>[4x]MKPLLSGSIPVEQFVQTLEKHGFSDIKVEDTAKGHIVLLQEAETLIQIEEDSTHIICDNDEMLRVRLRDLVLKFLQKF;>GSHMRLVSSEQA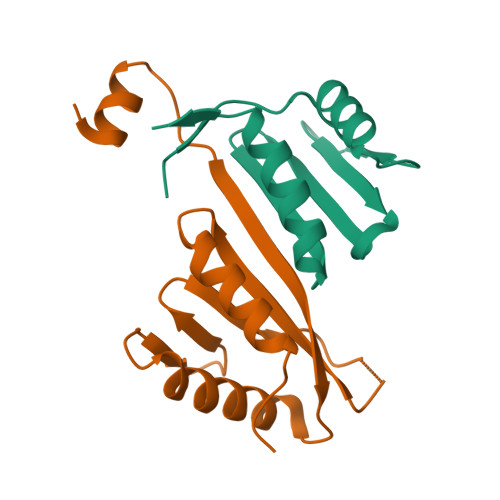LKELGLAEHQLRFTCRVHLHDTRKEQETALRVYSHLKSVLKDHCVQHLPDGSVTVESVLLQAAAPSEDPGTKVLLVSWTYQDEELGSFLTSLLKKGLPQAPS[4x]> GDPYWAYSGAYGPEHWVTSSVSCGGRHQSPIDILDQYARVGEEYQELQLDGFDNESSNKTWMKNTGKTVAILLKDDYFVSGAGLPGRFKAEKVEFHWGHSNGSAGSEHSINGRRFPVEMQIFFYNPDDFDSFQTAISENRIIGAMAIFFQVSPRDNSALDPIIHGLKGVVHHEKETFLDPFVLRDLLPASLGS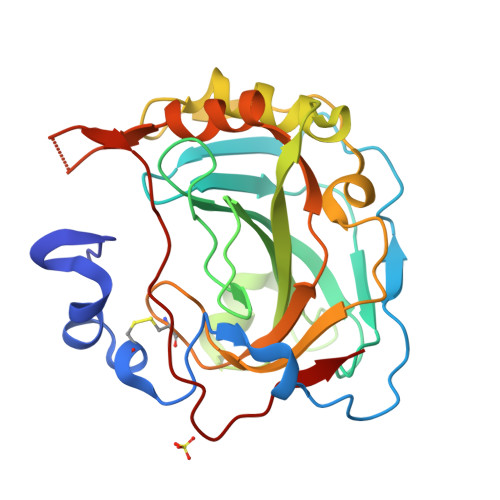YYRYTGSLTTPPCSEIVEWIVFRRPVPISYHQLEAFYSIFTTEQQDHVKSVEYLRNNFRPQQRLHDRVVSKS> SAKDFSGAELY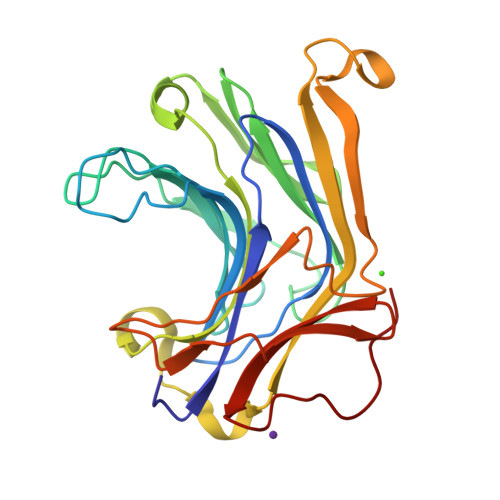TLEEVQYGKFEARMKMAAASGTVSSMFLYQNGSEIADGRPWVEVDIEVLGKNPGSFQSNIITGKAGAQKTSIKHHAVSPAADQAFHTYGLEWTPNYVRWTVDGQEVRKTEGGQVSNLTGTQGLRFNLWSSESAAWVGQFDESKLPLFQFINWVKVYKYTPGQGEGGSDFTLDWTDNFDTFDGSRWGKGDWTFDGNRVDLTDKNIYSRDGMLILALTRKGQESFNGQVPRD>GIDPFTADKGKCGLPEIFDPPEELERKVWELARLVWQSSSVVFHTGAGISTASGIPDFRGPHGVWTMEERGLAPKFDTTFESARPTQTHMALVQLERVGLL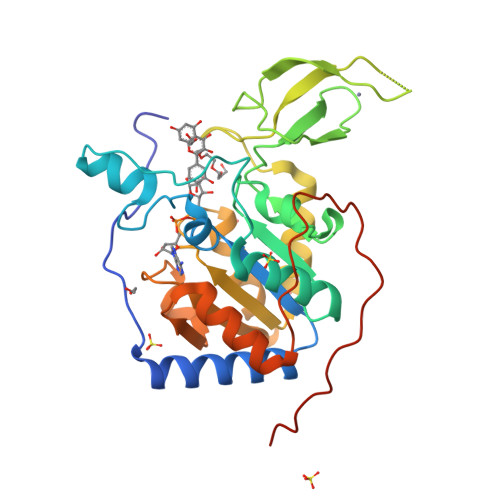RFLVSQNVDGLHVRSGFPRDKLAELHGNMFVEECAKCKTQYVRDTVVGTMGLKATGRLCTVAKARGLRACRGELRDTILDWEDSLPDRDLALADEASRNADLSITLGTSLQIRPSGNLPLATKRRGGRLVIVNLQPTKHDRHADLRIHGYVDEVMTRLMKHLGLEIPAWDGPRVLERALPPLPRPPTPKLEPKEESPTRIN[2x]Covalent DNA-protein crosslinks (DPCs) are toxic DNA lesions that interfere with essential chromatin transactions, such as replication and transcription. In yeast, DPC proteolysis is catalyzed by the metalloprotease Wss1, which permits replication in the presence of DPCs and provides resistance toward DPC-inducing agents. Intriguingly, Wss1 is a DNA-dependent protease that degrades DNA-bound substrates in vitro irrespective of identity. Spartan (SPRTN, DVC1) is distantly related to yeast Wss1, displays a similar domain organization, and shares a common evolutionary origin (Stingele et al., 2015).

While most proteins were insoluble, we were able to purify the protease domain of Wss1b, one of the two SPRTN homologs in Schizosaccharomyces pombe. The overall architecture depicted a compact protease domain consisting of four tightly packed α helices and a four-stranded antiparallel β sheet. The glutamate residue E112 polarized a water molecule for the nucleophilic attack of the substrate; in agreement, its mutation to glutamine resulted in a catalytically inactive enzyme.

>GSIYTFNELVVLDYPHKDRALRYLERLRDDTGIKKIMDSHRWTVPLLSEMDPAEHTRHDSKTLGLNHNQGAHIELRLRTDRYDGFRDYKTVKSTLIHQLTHNVHGEHDSSFWELFRQLTKEADAADLL[2x]>MSNEVEQKKNIKTINDLPGISQTVINKLIEAGYSSLETLAVASPQDLSVAAGIPLSTAQKIIKEARDALDIRFKTALEVKKERMNVKKISTGSQALDGLLAGGIETRTMTEFFGEFGSGKTQLCHQLSVNVQLPPEKGGLSGKAVYIDTEGTFRWERIENMAKALGLDIDNVMNNIYYIRAINTDHQIAIVDDLQELVSKDPSIKLIVVDSVTSHFRAEYPGRENLAVRQQKLNKHLHQLTRLAEVYDIAVIITNQVMARPD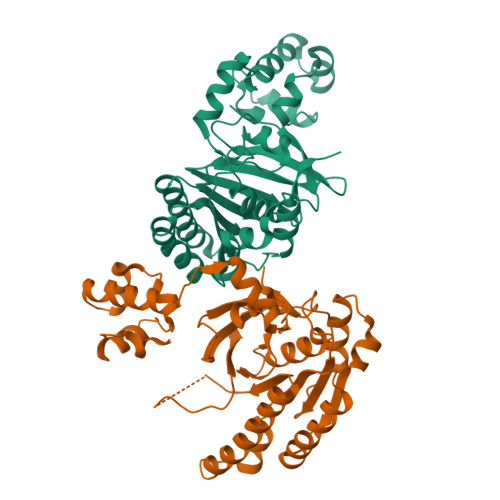MFYGDPTVAVGGHTLYHVPGIRIQLKKSRGNRRIARVVDAPHLPEGEVVFALTEEGIRDAEE[2x]METHANETHIOL | C 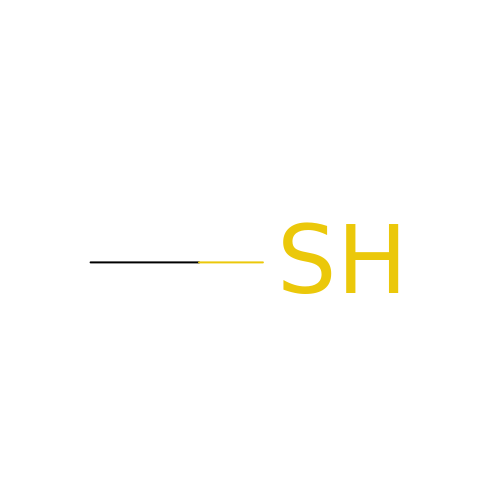H4 S | LSDPWZHWYPCBBB-UHFFFAOYSA-N Members of the ring-forming Hsp104/ClpB family of ATP-driven molecular chaperones are the principle protein disaggregases in fungi (Hsp104), plants (Hsp101), and eubacteria (ClpB). At the molecular level, Saccharomyces cerevisiae Hsp104 forms a homo-hexamer that is stabilized by adenine nucleotides. Each Hsp104 monomer features two ATP-binding domains, termed AAA-1 and AAA-2, in addition to an N-terminal (N) domain and a coiled-coil motif that mediates the physical interaction with Hsp70. It is now widely accepted that Hsp104 facilitates the unfolding of aggregated proteins and the threading of substrate through the protein translocation channel analogous to ATP-dependent Clp proteases.

Here we present the orthorhombic crystal structure of an N-terminal fragment of S. cerevisiae Hsp104 (Hsp1041-360) comprising the N domain (residues 4–164), the AAA-1large domain (residues 165–341), and the first α-helix of the AAA-1small domain (residues 345–356). The structure of Hsp1041-360 was determined by molecular replacement and was refined to a resolution of 2.6 Å. We did not observe any unaccounted electron density that could be attributed to a bound nucleotide, even when 5 mM nucleotide (ADPNP or ADP) was added for crystallization, indicating that Hsp1041-360 was crystallized in the nucleotide-free state. The crystal structure consists of three Hsp1041-360 monomers (mol 1, mol 2, and mol 3) that are structurally independent and in different physicochemical environments, which allows the identification of common structural features that may be of functional importance. Superimposing the crystal structures of the complete Hsp1041-360 fragment through their AAA-1large domain shows that the orientation of the N domain seen in mol 1 and mol 2 is rotated by 172–174° relative to that in mol 3 with residues 161–165 making up the hinge region. The first AAA-1 pore loop (loop-1), comprising residues 253–259, is seen in all three monomers, and loop-2, comprising residues 291–294, is ordered in two molecules. In our structure, Tyr257 makes contact with the N domain of a neighboring, non-crystallographic symmetry (NCS) related molecule. In addition, the aliphatic side chain of Lys256 forms a stacking interaction with the Tyr257 side chain, which may orient Tyr257, while the ε-amino group of Lys256 makes an ionic interaction with the Glu146 side chain of a neighboring molecule. In our structure, loop-2 adopts two distinct conformations in an ‘up’ and ‘down’ configuration when viewed along the six-fold axis of the Hsp104 hexamer. Residue 292 (asparagine) that is non-conserved in ClpA/B proteins, is in van der Waals contact with the N domain of an NCS-related, neighboring molecule (Lys131), resembling an interaction with substrate.

>[3x]QTQFTERALTILTLAQKLASDHQHPQLQPIHILAAFIETPEDGSVPYLQNLIEKGRYDYDLFKKVVNRNLVRIPQQQPAPAEITPSYALGKVLQDAAKIQKQQKDSFIAQDHILFALFNDSSIQQIFKEAQVDIEAIKQQALELRGNTRIDSRGADTNTPLEYLSKYAIDMTEQARQGKLDPVIGREEEIRSTIRVLARRIKSNPCLIGEPGIGKTAIIEGVAQRIIDDDVPTILQGAKLFSLDLAALTAGAKYKGDFEERFKGVLKEIEESKTLIVLFIDEIHMLMGNGKDDAANILKPALSRGQLKVIGATTNNEYRSIVEKDGAFERRFQKIEVAEPSVRQTVAILRGLE>[2x]MRYIVALTGGIGSGKSTVANAFADLGINVIDADIIARQVVEPGAPALH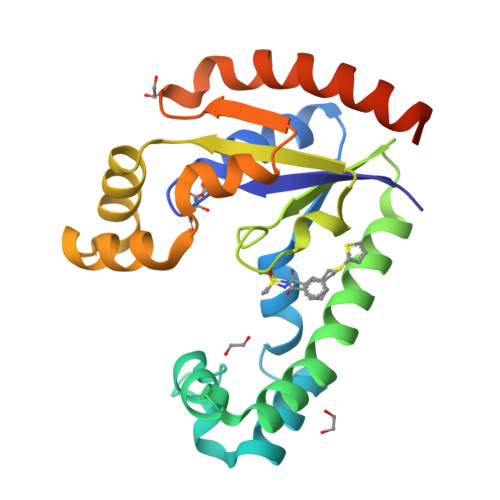AIADHFGANMIAADGTLQRRALRERIFANPEEKNWLNALLHPLIQQETQHQIQQATSPYVLWVVPLLVENSLYKKANRVLVVDVSPETQLKRTMQRDDVTREHVEQILAAQATREARLAVADDVIDNNGAPDAIASDVARLHAHYLQLASQFVSQEKPGSHHHHHH> GHMSEHVHKELLHLGEVFRSQREERALSLKDVE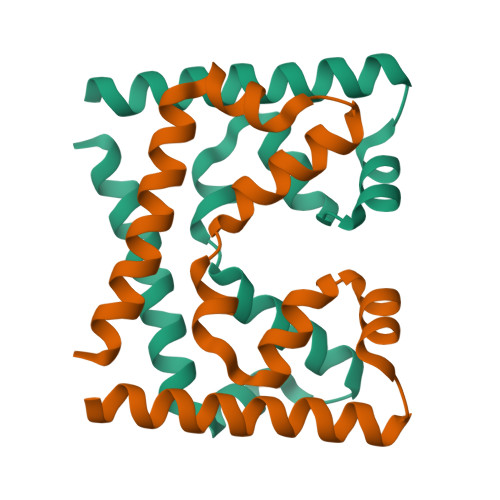AATSIRLSALEAIEAGHLGKLISPVYAQGFMKKYAAFLDMDGDRLLKEHPYVLKIFQEFSDQNMDMLLDLESMGGRNSPEKAIRS> GSHMASPNGQTKPLPALKLALEYIVPCMNKHGICVVDDFLGKETGQQIGDEVRALHDTGKFTDGQLVSQKSDSSKDIRGDKITWIEGKEPGCETIGLLMSSMDDLIRHCNGKLGSYKINGRTKAMVACYPGNGTGYVRHVENPNGDGRCVTCIYYLNKDWDAKVSGGILRIFPEGKAQFADI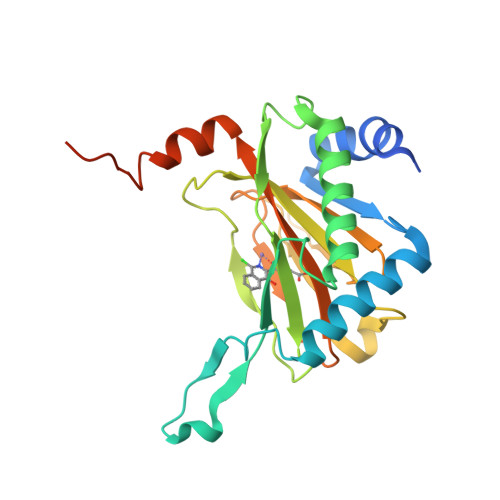EPKFDRLLFFWSDRRNPHEVQPAYATRYAITVWYFDADERARAKVKYLTGEKGVRVELNKPSDSVGKDVF> KPKGHPHMNSIRIDGDITLGGLFPVHGRGSEGKPCGELKKEKGIHRLEAMLFALDRINNDPDLLPNITLGARILDTCSRDTHALEQSLTFVQALIEKDGTEVRCGSGGPPIITKPERVVGVIGASGSSVSIMVANILRLFKIPQISYASTAPDLSDNSRYDFFSRVVPSDTYQAQAMVDIVRALKWNYVSTVASEGSYGESGVEAFIQKSREDGGVCIAQSVKIPREPKAGEFDKIIRRLLETSNARAVIIFANEDDIRRVLEAARRANQTGHFFWMGSDSWGSKIAPVLHLEEVA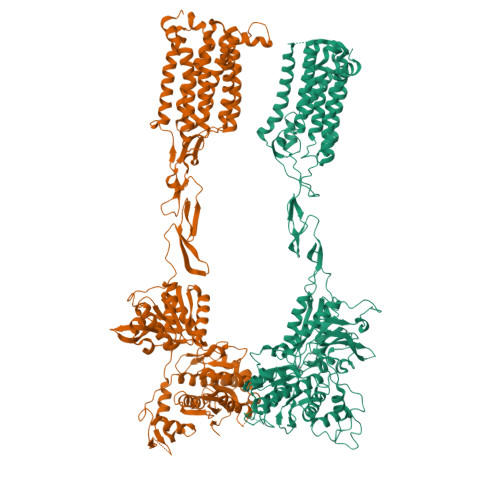EGAVTILPKRMSVRGFDRYFSSRTLDNNRRNIWFAEFWEDNFHCKLSRHALKKGSHVKKCTNRERIGQDSAYEQEGKVQFVIDAVYAMGHALHAMHRDLCPGRVGLCPRMDPVDGTQLLKYIRNVNFSGIAGNPVTFNENGDAPGRYDIYQYQLRNDSAEYKVIGSWTDHLHLRIERMHWPGSGQQLPRSICSLPCQPGERKKTVKGMPCCWHCEPCTGYQYQVDRYTCKTCPYDMRPTENRTGCRPIPIIKLEWGSPWAVLPLFLAVVGIAATLFVVITFVRYNDTPIVKASGRELSYVLLAGIFLCYATTFLMIAEPDLGTCSLRRIFLGLGMSISYAALLTKTNRIYRIFEQGKRSVSAPRFISPASQLAITFSLISLQLLGICVWFVVDPSHSVVDFQDQRTLDPRFARGVLKCDISDLSLICLLGYSMLLMVTCTVYAIKTRGVPETFNEAKPIGFTMYTTCIVWLAFIPIFFGTSQSADKLYIQTTTLTVSVSLSASVSLGMLYMPKVYIILFHPEQNVPKRKRSLKAVVTAATMSNKFTQKGNFRPNGEAKSELCENLEAPALATKQTYVTYTNHAI;> EGPAKKVLTLEGDLVLGGLFPVHQKGGPAEDCGPVNEHRGIQRLEAMLFALDRINRDPHLLPGVRLGAHILDSCSKDTHALEQALDFVRASLSRGADGSRHICPDGSYATHGDAPTAITGVIGGSYSDVSIQVANLLRLFQIPQISYASTSAKLSDKSRYDYFARTVPPDFFQAKAMAEILRFFNWTYVSTVASEGDYGETGIEAFELEARARNICVATSEKVGRAMSRAAFEGVVRALLQKPSARVAVLFTRSEDARELLAASQRLNASFTWVASDGWGALESVVAGSEGAAEGAITIELASYPISDFASYFQSLDPWNNSRNPWFREFWEQRFRCSFRQRDCAAHSLRAVPFEQESKIMFVVNAVYAMAHALHNMHRALCPNTTRLCDAMRPVNGRRLYKDFVLNVKFDAPFRPADTHNEVRFDRFGDGIGRYNIFTYLRAGSGRYRYQKVGYWAEGLTLDTSLIPWASPSAGPLPASRCSEPCLQNEVKSVQPGEVCCWLCIPCQPYEYRLDEFTCADCGLGYWPNASLTGCFELPQEYIRWGDAWAVGPVTIACLGALATLFVLGVFVRHNATPVVKASGRELCYILLGGVFLCYCMTFIFIAKPSTAVCTLRRLGLGTAFSVCYSALLTKTNRIARIFGGAREGAQRPRFISPASQVAICLALISGQLLIVVAWLVVEAPGTGKETAPERREVVTLRCNHRDASMLGSLAYNVLLIALCTLYAFKTRKCPENFNEAKFIGFTMYTTCIIWLAFLPIFYVTSSDYRVQTTTMCVSVSLSGSVVLGCLFAPKLHIILFQPQKNVVSHRAPTSRFGSAAARASSSLGQGSGSQFVPTVCNGREVVDSTTSSL> SQGVIGIFGDYAK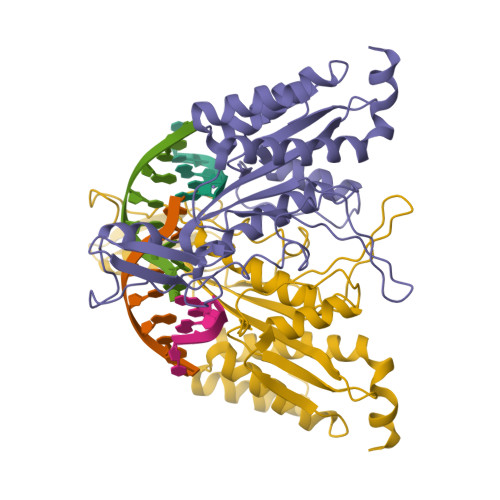AHDLAVGEVSKLVKKALSNEYPQLSFRYRDSIKKTEINEALKKIDPDLGGTLFVSNSSIKPDGGIVEVKDDYGEWRVVLVAEAKHQGKDIINIRNGLLVGKRGDQDLMAAGNAIERSHKNISEIANFMLSESHFPYVLFLEGSNFLTENISITRPDGRVVNLEYNSGILNRLDRLTAANYGMPINSNLCINKFVNHKDKSIMLQAASIYTQGDGREWDSKIMFEIMFDISTTSLRVLGRDLFEQLTSK>MGHHHHHHGSDPNEAVREFAKEIDVSFVKIEEVIGAGEFGEVYKGRLKLPGKREIYVAIKTLKAGYSEKQRRDFLSEASIMGQFDHRNIIRLEGVVTKSRPVMIITEFMENGALDSFLRQNDGQFTVIQLVGMLRGIAAGMKYLSEMNYVHRDLAARNILVNSNLVCKVSDFGLSRYLQDDTSDPTYTSSLGGKIPVRWTAPEAIAYRKFTSASDVWSYGIVMWEVMSFGERPYWDMSNQDVINAIEQDYRLPPPMDCPAALHQLMLDCWQKDRNSRPRFAEIVNTLDKMIRNPASLKTVATITA[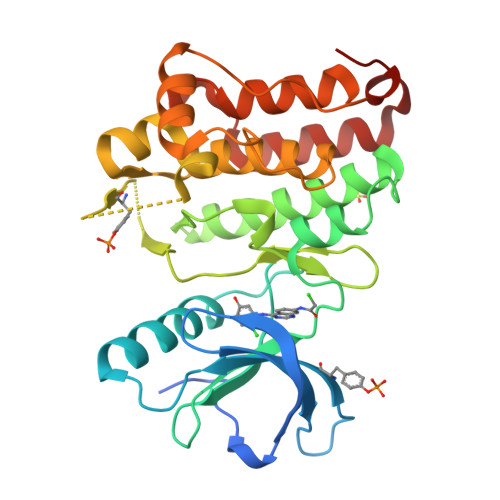2x]>G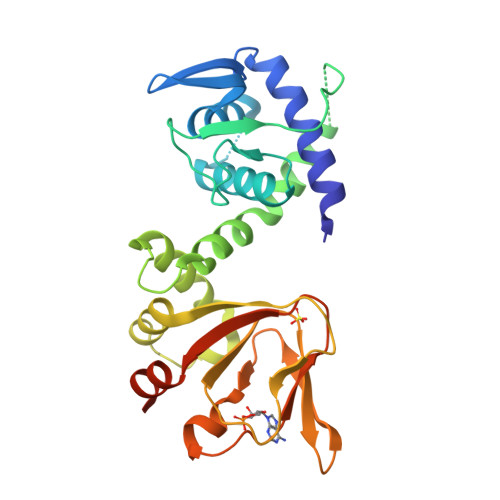ASTERVLRAGRQLHRHLLATCPNLIRDRKYHLRLYRQCCSGRELVDGILALGLGVHSRSQVVGICQVLLDEGALCHVKHDWAFQDRDAQFYRFPGPEPEPVGTHEMEEELAEAVALLSQRGPDALLTVALRKPPGQRTDEELDLIFEELLHIKAVAHLSNSVKRELAAVLLFEPHSKAGTVLFSQGDKGTSWYIIWKGSVNVVTHGKGLVTTLHEGDDFGQLALVNDAPRAATIILREDNCHFLRVDKQDFNRIIKDVEAKTMRLEEHG[2x]> MGRDPNSTNDTTTQNVVLTKYGFDKDVTAIDRATDQIWTGDGAKPLQGVDFTIYNVTANYWASPKDYKGSFDSAPVAATGTTNDKGQLTQALPIQSKDA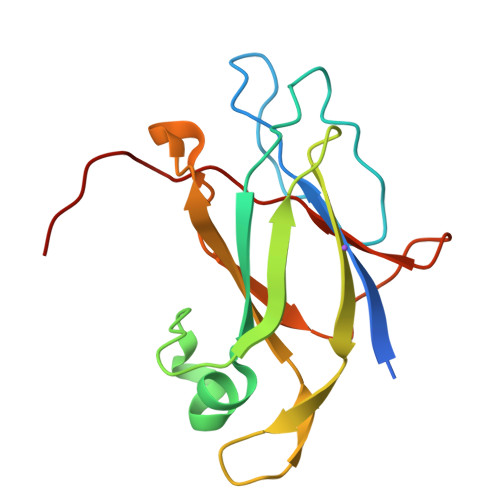SGKTRAAVYLFHETNPRAGYNTSADFWLTLPAKAAADGNVYVYPKNVQKTTYER>[3x]MSFFHASQRDALNQSLAEVQGQINVSFQFFPPRTSEMEQTLWNSIDRLSSLKPKFVSVTYGANSGERDRTHSIIKGIKDRTGLEAAPHLTCIDATPDELRTIARDYWNNGIR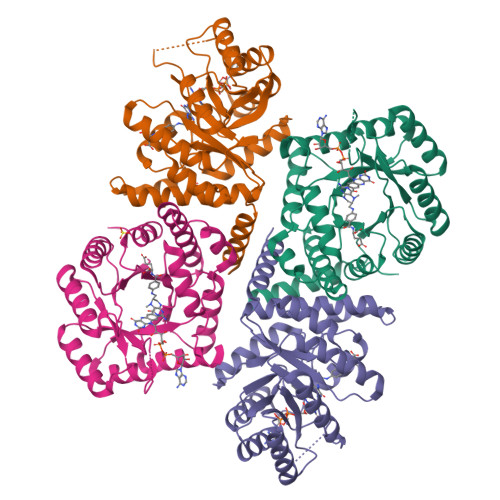HIVALRGDLPPGSGKPEMYASDLVTLLKEVADFDISVAAYPEVHPEAKSAQADLLNLKRKVDAGANRAITQFFFDVESYLRFRDRCVSAGIDVEIIPGILPVSNFKQAKKFADMTNVRIPAWMAQMFDGLDDDAETRKLVGANIAMDMVKILSREGVKDFHFYTLNRAEMSYAICHTLGVRPGLLEHHHHHH To understand the molecular basis underlying the superbinding characteristics of the Legionella SH2 domains, we determined the structures of L. longbeachae LeSH and the L. pneumophila RavO SH2 domain in complex with tyrosine-phosphorylated peptides by X-ray crystallography. Compared to the Src SH2 domain, LeSH is missing two β-strands (βA and βF) but contains a 45-residue insert between the strand βE and the helix αB. This extra sequence in LeSH contains a structural motif called the pancreatic polypeptide (PP)-fold, comprising an amphipathic α-helix (named herein as αEF) packed against a polyproline segment via favorable hydrophobic contacts. Indeed, the SH2 and PP folds together form a clamp-like structure that grasp the pTyr residue.

Therefore, LeSH may be considered a hybrid of two eukaryotic protein folds – SH2 and PP. Because the PP-fold occupies the same position as the EF loop in a eukaryotic SH2 domain, they may play a similar role in ligand binding. An overlay of the LeSH structures in apo and peptide-bound forms identified the PP-fold as the only region in LeSH that undergoes a significant conformational change upon peptide binding. Molecular simulation suggested that the motion of the PP-fold was distinct from that of the SH2 fold. Therefore, it is likely that the pTyr-clamp in LeSH may be able to adjust its conformation to a certain degree to accommodate different peptides. This mechanism of ligand binding may be employed by other Legionella SH2 domains of the LeSH subfamily.

> GAMEAMQKNELNSKIPIIFGLINSYQIHNLLEQHNAKTKESKAVFLIRDSSTYPGLLTISYYCQEQDIVKHIRFGLTDKGWKTAPKPPHEPLKSDSPEIKEKYTLDKIKFERKMKQFINTAKKLFEQHIRAESFKTLIMELKIHEFNLEGLIKPTRSQASQEKHFTDYV>MEKDRKRILITGGAGFVGSHLTDKLMMDGHEVTVVDNFFTGRKRNVEHWIGHENFELINHDVVEPLYIEVDQIYHLASPASPPNYMYNPIKTLKTNTIGTLNMLGLAKRVGARLLLASTSEVYGDPEVHPQSEDYWGHVNPIGPRACYDEGKRVAETMCYAYMKQEGVEVRVARIFNTFGPRMHMNDGRVVSNFILQALQGEPLTVYGSGSQTRAFQYVSDLVNGLVALMNSNVSSPVNLGNPEEHTILEFAQLIKNLVGSGSEIQFLSEAQDDPQ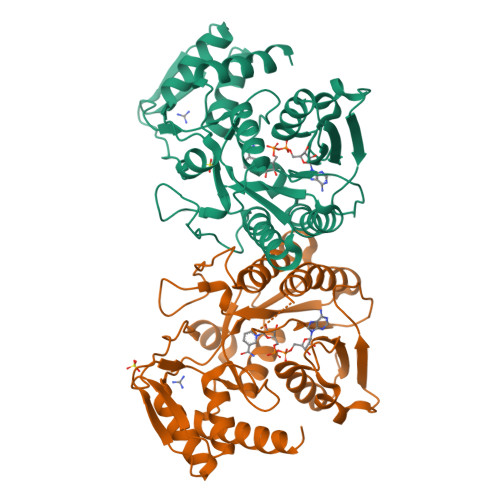KRKPDIKKAKLMLGWEPVVPLEEGLNKAIHYFRKELEYQANNQYIPKPKPARIKKGRTRHS[2x]>[2x]GGGGGGHMKIIIAGKNDIAVNVTRWLQKKKKNIEIYAICNANDTGIDTFQRSFKKYCKDNLIPIISLAEAYKIDDAIFLSLEFDKIVQPSKFNHNELFNIHFSYLPKYKGMYTSAWPILNGEDTSGVTLHKIDHGIDTGAIIAQKEIIIQPFETAKDLYEKYISEGTSLVIDNISTLLNSEYVEKEQNIKYSSYYSKKTIDYSNLELNFSKTAFEIINQLRAFTFREYQLPKLDGVNIFLGDVLS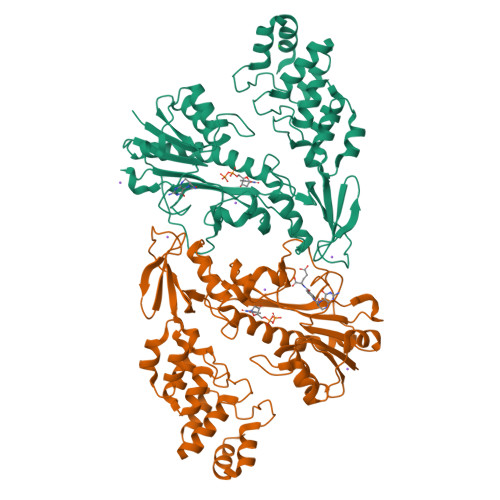SRSIMKPGSILERNDKEIIVSTIDYDVVLYKDNFKEILEACKYSDSKYIAKLIRAKSILFEKNIYGASPVIVAAYHGNIELIKWLVSKGANINDRNYKGTTVAMYFKDYMLKSGDYSGLKMLIDLGLDLTLTDYKDYTVFDYLEKSGNKNLLQYMMAFMK> MLQNSFKLAQSLRNGFYRNAWRAFSSHGPRQPLVSPERRLEKAHPTFTERSQLKYARRLVVKLGSAVITREDNHGLALGRLASIVEQVAECHLEGREVMMVTSGAVAFGKQKLAQELLMSLSMRETLNPKDSKEFDGATLEPRAAAAVGQSGLMSLYDAMFAQYGVKIAQVLVTKPDFYNEETRNNLFCTLSELISLNIVPIINTNDAVSPPMFIRDDEPAGGARRGIPIKDNDSLSAMLAAEVQADLLILMSDVDGIYNKPPWEDGAKLMHTYTSDDSNSIEFGKKSKVGTGGMDSKVKAATWALDRGVSVVICNGMQEKAIKTIIGGRKVGTFFTEATESANAVPVEVMAENARTGSRQMQALTPAQRASAVNTLADLLVSREKFILDANAKDLAEAQKSGLAKPLLSRLSLNPAKLKNLSVGLKQIAEDSHKNVGRVLRRTRLADQLELKQVTVPIGVLLVIFESRPDSLPQVAALAMASANGLLLKGGKEAAHSNKALMELVKEALATVGAEHAVSLVSTREEISDLLSMENHIDLIIPRGSSDLVRSIQQQSLHIPVLGHAEGVCHVYIDRDADLEKALRIARDAKCDYPAACNAMETLLIHEDLMSGAIFGDVCNMLKREGVKIYAGPRLNQQLT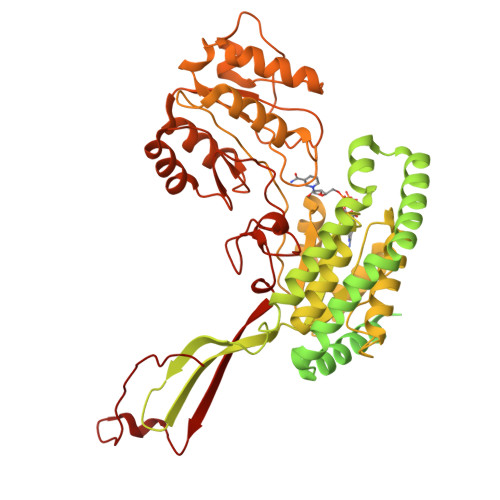FGPPAAKSLKHEYGALECCIEVVPSLDEAINHIHTYGSSHTDVIVTENDAAARQFLGSVDSACVFHNASSRFADGFRFGLGAEVGISTARIHARGPVGVEGLLTTKWILEGQDHAAADFAEGGGRTWLHETLPLD> EQSSSEIKIVRDEYGMPHIYANDTWHLFYGYGYVVAQDRLFQMEMARRSTQGTVAEVLGKDFVKFDKDIRRNYWPDAIRAQIAALSPEDMSILQGYADGMNAWIDKVNTNPETLLPKQFNTFGFTPKRWEPFDVAMIFVGTMANRFSDSTSEIDNLALLTALKDKYGVSQGMAVFNQLKWLVNPSAPTTIAVQESNYPLKFNQQNSQTA;> SNMWVIGKSKAQDAKAIMVNGPQFGWYAPAYTYGIGLHGAGYDVTGNTPFAYPGLVFGHNGVISWGSTAGFGDDVDIFAERLSAEKPGYYLHNGKWVKMLSREETITVKNGQAETFTVWRTVHGNILQTDQTTQTAYAKSRAWDGKEVASLLAWTHQMKAKNWQEWTQQAAKQALTINWYYADVNGNIGYVHTGAYPDRQSGHDPRLPVPGTGKWDWKGLLPFEMNPKVYNPQSGYIANWNNSPQKDYPASDLFAFLWGGADRVTEIDRLLEQKPRLTADQAWDVIRQTSRQDLNLRLFLPTLQAATSGLTQSDPRRQLVETLTRWDGINLLNDDGKTWQQPGSAILNVWLTSMLKRTVVAA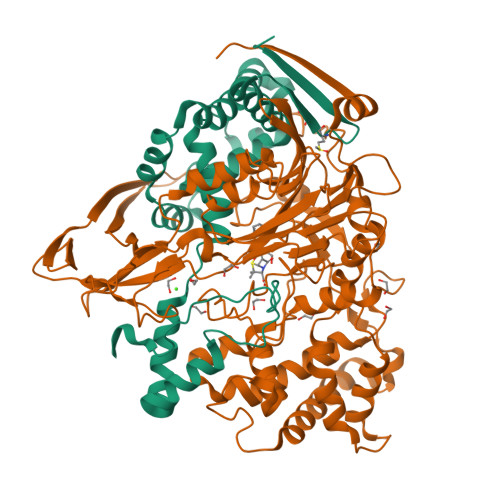VPMPFDKWYSASGYETTQDGPTGSLNISVGAKILYEAVQGDKSPIPQAVDLFAGKPQQEVVLAALEDTWETLSKRYGNNVSNWKTPAMALTFRANNFFGVPQAAAEETRHQAEYQNRGTENDMIVFSPTTSDRPVLAWDVVAPGQSGFIAPDGTVDKHYEDQLKMYENFGRKSLWLTKQDVEAHKESQEVLHVQR>[4x]SNAEYDLFISHASEDKEDFVRPLAETLQQLGVNVWYDEFTLK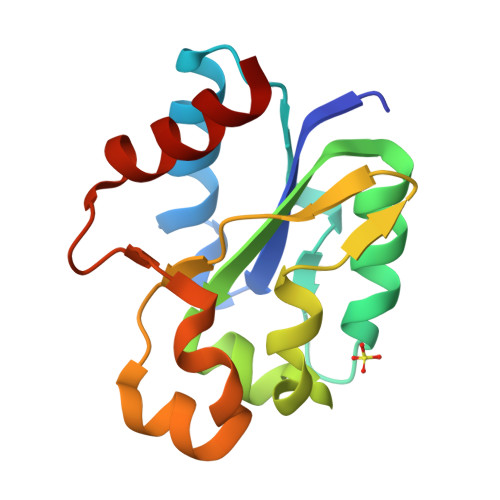VGDSLRQKIDSGLRNSKYGTVVLSTDFIKKDWTNYELDGLVAREMNGHKMILPIWHKITKNDVLDYSPNLADKVALNTSVNSIEEIAHQLADVIL>MSPISRHHHHHHLVPRGSASLRANDAPIVLLHGFTGWGREEMFGFKYWGGVRGDIEQWLNENGYRTYTLAVGPLSSNWDRACEAYAQLVGGTVDYGAAHAAKHGHARFGRTYPGLLPELKRGGRIHIIAHSQGGQNARMLVSLLENGSQEEREYAKAHNVSLSPLFEGGHHFVLSVTTIATPHDGTTLVNMVDFTDRFFDLQKAVLEAAAVASNVPYTSQVYDFKLDQWGLRRQPGESFDHY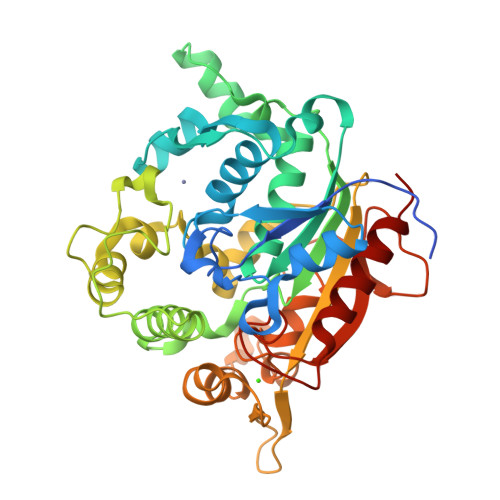FDRLKRSPVWTSTDTARYDLSVSGALKLNQWVQASPNTYYLSFSTERTYRGALTGNHYPELGMNAFSAVVCAPFLGSYREPTLGIDDRWLENDGIVNTVSMNGPKRGSSDRIVPYDGTLKKGVWNDMGTYNVDHLEIIGVDPNPSFDIRAFYLRLAEQLASLRP[2x]> MELRDRIDFLCKTILAIKTAGRLVLGIDGLSRSGKTTLANQLSQTLREQGISVCVFHMDDHIVERAKRYHTGNEEWFEYYYLQWDVEWLTHQLFRQLKASHQLTLPFYDHETDTHSKRTVYLSDSD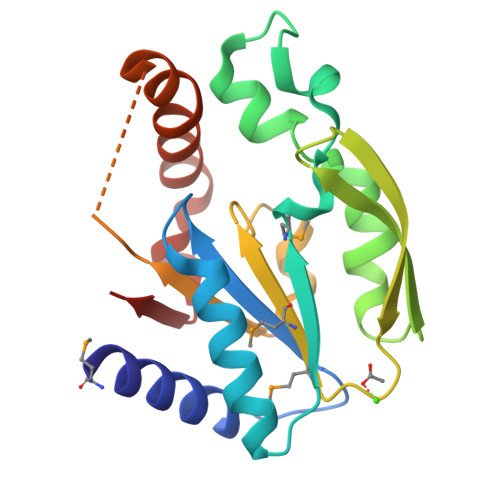MIMIEGVFLQRKEWRPFFDFVVYLDCPREIRFARENDQVKQNIQKFINRYWKAEDYYLETEEPIKRADVVFDMTS NoV VP1 has two principle domains, the shell (S) and the protruding (P) domains, linked by a short, flexible hinge. The S domain builds the interior shell that forms the basic structure of the icosahedral capsid, while the P domain dimerizes constituting the arch-like protrusions extending from the shell. HuNoVs recognize histo-blood group antigens (HBGAs) as attachment factors or receptors which play an important role in the host susceptibility to huNoV infections. BV, a clinical isolate, bound uniquely to the Le, but not the A and H antigens, making the BV distinct from other tested GI NoVs that bind generally the A and H antigens.

The native BV P protein was crystallized under the space group of P61, containing two P protein protomers in an asymmetric unit, related by a non-crystallographic 2-fold axis. Peptide chain ranging from K230 to L526 can be modeled, while distal parts of two loop regions in the P1 subdomain (see below) comprising Q260/N261 and G502/G503, respectively, could not be modeled due to un-interpretable local electron density maps. As expected, the P protein is dimerized via a non-crystallographic 2-fold axis, forming an arch-like P dimer in dimension of 54 Å × 62 Å × 67 Å. The P dimer is stabilized by the vast monomer buried surface area of 3,733 Å2 (including two monomers) comprised of both hydrophobic and hydrophilic residue interactions contributed from both P1 and P2 subdomains. BV P domain retains the basic structures of the GI NoV P domains. The P1 subdomain, constituted by the N′ (K230–A279) and C′ (A420–L526) terminal regions, forms mainly the legs of the arch-like P dimer (see below), while the P2 subdomain, formed by a large insertion from R280 to L419, builds the majority of the head of the P dimer. The P1 subdomain is a mixed α/β structure containing an amphiphile α helix and two twisted antiparallel β sheets: β1-β9-β10 and β9-β11-β12-β13-β14, where β9 strand was shared between the two β sheets. The P2 subdomain is constituted mainly by a β-barrel structure formed by two twisted antiparallel β sheets: β5-β4-β8 and β8-β2-β3-β7-β6. The major structural differences among the four P domains reside on 6 loop regions, including the previously identified A-, B-, P-, T- and U-loops in the P2 subdomain and the S-loop in the P1 subdomain, consistent with the variations, insertions and/or deletions of the sequences of the loops. The five loops (A-, B-, P- S- and T-loops) occupy the majority of the top surface of the BV P dimer. In contrast, the S- and T-loops become shorter and less exposed in BV compared with other three GI counterparts.

>GPLGSPEFQRTKPFSVPNIPMNLMSNSRVPMLIDGMMVSNDQNQVPQFQNGRVTLDGQLQGTTTVSAACIARMRGRIFNNNGNYGVNLAELDGNPYHAFDSPAPLGFPDFGNCDLHMTFVKINPTELSTGDPSGKVVIHSYDATFAPHLGTVKLEDNNELDQFVGKEVVLELTWVSNRTGATLNLWAVPNYGSNLTQASQLAPPIYPPGFGEAIVYFTSTFPTVSNPKVPCTLPQEFVSHFVNEQAPTRGDAALLHYVDPDTHRNLGEFKMYPEGYMTCVPNAGGGPQTLPINGVFVFISWVSRYYQL[2x]> GTSTQTKAGSLTIVGTGIESIGQMTLQALSYIEAAAKVFYCVIDPATEAFILTKNKNCVDLYQYYDNGKSRLNTYTQMSELMVREVRKGLDVVGVFYGHPGVFVNPSHRALAIAKSEGYRARMLPGVSAEDCLFADLCIDPSNPGCLTYEASDFLIRDRPVSIHSHLVLFQVGCVGIADFNFT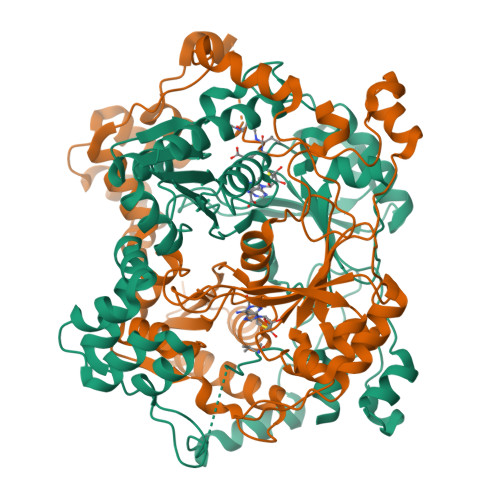GFDNNKFGVLVDRLEQEYGAEHPVVHYIAAMMPHQDPVTDKYTVAQLREPEIAKRVGGVSTFYIPPKARKASNLDIIRRLELLPAGQVPDKKARIYPANQWEPDVPEVEPYRPSDQAAIAQLADHAPPEQYQPLATSKAMSDVMTKLALDPKALADYKADHRAFAQSVPDLTPQERAALELGDSWAIRCAMKNMPSSLLDAARESGEEASQNGFPWVIVEGVIGVIGSVMSTE;> GTSTQTKAGSLTIVGTGIESIGQMTLQALSYIEAAAKVFYCVIDPATEAFILTKNKNCVDLYQYYDNGKSRLNTYTQMSELMVREVRKGLDVVGVFYGHPGVFVNPSHRALAIAKSEGYRARMLPGVSAEDCLFADLCIDPSNPGCLTYEASDFLIRDRPVSIHSHLVLFQVGCVGIADFNFTGFDNNKFGVLVDRLEQEYGAEHPVVHYIAAMMPHQDPVTDKYTVAQLREPEIAKRVGGVSTFYIPPKARKASNLDIIRRLELLPAGQVPDKKARIYPANQWEPDVPEVEPYRPSDQAAIAQLADHAPPEQYQPLATSKAMSDVMTKLALDPKALADYKADHRAFAQSVPDLTPQERAALELGDSWAIRCAMKNMPSSLLDAARESGEEASQNGFPWVIVXGVIGVIGSVMSTE> GAADKGEIRVGNRYQADITDLLKEGEEDGRDQSRLETQVWEAHNPLTDKQIDQFLVVARSVGTFARALDCSSSVRQPSLHMSAAAASRDITLFHAMDTLHKNIYDISKAISALVPQGGPVLCRDEMEEWS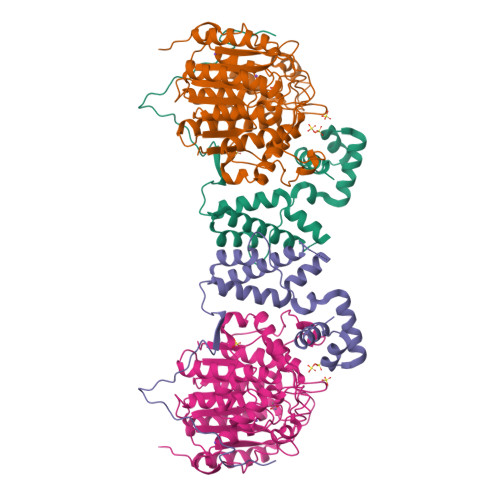ASEANLFEEALEKYGKDFTDIQQDFLPWKSLTSIIEYYYMWKTTDR;> MAQTQGTRRKVCYYYDGDVGNYYYGQGHPMKPHRIRMTHNLLLNYGLYRKMEIYRPHKANAEEMTKYHSDDYIKFLRSIRPDNMSEYSKQMQRFNVGEDCPVFDGLFEFCQLSTGGSVASAVKLNKQQTDIAVNWAGGLHHAKKSEASGFCYVNDIVLAILELLKYHQRVLYIDIDIHHGDGVEEAFYTTDRVMTVSFHKYGEYFPGTGDLRDIGAGKGKYYAVNYPLRDGIDDESYEAIFKPVMSKVMEMFQPSAVVLQCGSDSLSGDRLGCFNLTIKGHAKCVEFVKSFNLPMLMLGGGGYTIRNVARCWTYETAVALDTEIPNELPYNDYFEYFGPDFKLHISPSNMTNQNTNEYLEKIKQRLFENLRMLPHAPGVQMQAIPEDAIPEESGDEDEDDPDKRISICSSDKRIACEEEFSDSEEEGEGGRKNSSNFKKAKRVKTEDEKEKDPEEKKEVTEEEKTKEEKPEAKGVKEEVKLA2-(5-CARBAMIMIDOYL-2-HYDROXY-BENZYLAMINO)-PROPIONIC ACID | C11 H15 N3 O3 | 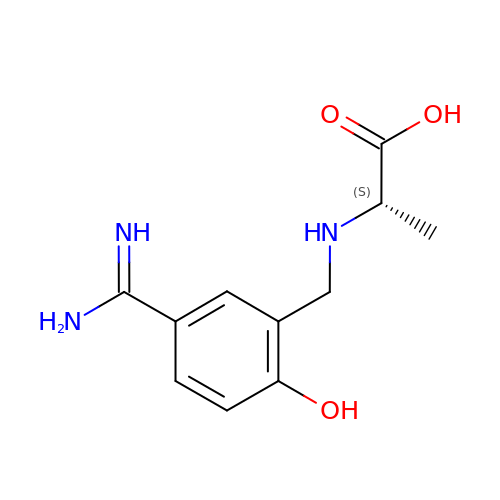CUGPJCUEKAARCR-LURJTMIESA-N>MFEQRVNSDVLTVSTVNSQDQVTQKPLRDSVKQALKNYFAQLNGQDVNDLYELVLAEVEQALLDMVMQYTRGNQTRAALMMGINRGTLRKKLKKYGMN[2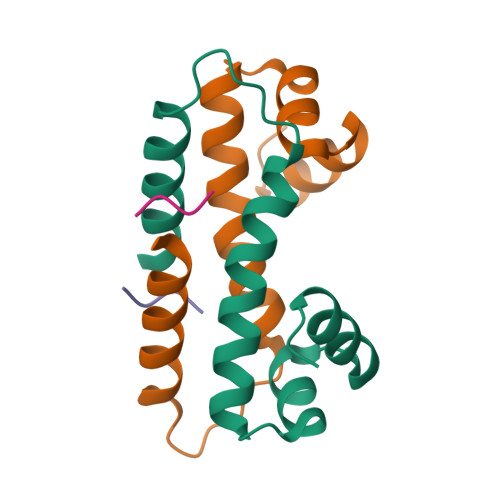x]> MHHHHHHHDGTEDPIHDRTSDYHKYLKVKQGDSDLFKLTVSDKRYIWYNPDPKERDSYECGEIVSETSDSFTFKTVDGQDRQVKKDDANQRNPIKFDGVEDMSELSYLNEPAVFHNLRVRYNQ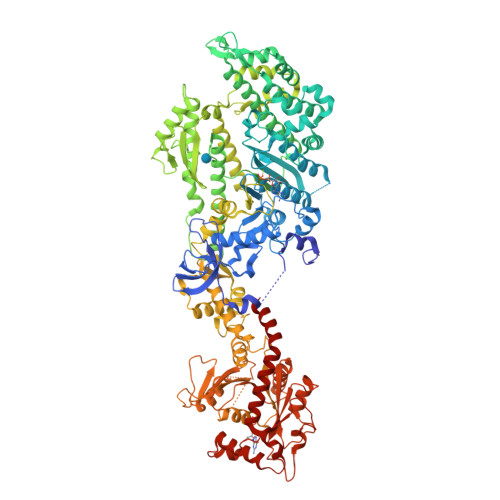DLIYTYSGLFLVAVNPFKRIPIYTQEMVDIFKGRRRNEVAPHIFAISDVAYRSMLDDRQNQSLLITGESGAGKTENTKKVIQYLASVAGRNQANGSGVLEQQILQANPILEAFGNAKTTRNNNSSRFGKFIEIQFNSAGFISGASIQSYLLEKSRVVFQSETERNYHIFYQLLAGATAEEKKALHLAGPESFNYLNQSGCVDIKGVSDSEEFKITRQAMDIVGFSQEEQMSIFKIIAGILHLGNIKFEKGAGEGAVLKDKTALNAASTVFGVNPSVLEKALMEPRILAGRDLVAQHLNVEKSSSSRDALVKALYGRLFLWLVKKINNVLCQERKAYFIGVLDISGFEIFKVNSFEQLCINYTNEKLQQFFNHHMFKLEQEEYLKEKINWTFIDFGLDSQATIDLIDGRQPPGILALLDEQSVFPNATDNTLITKLHSHFSKKNAKYEEPRFSKTEFGVTHYAGQVMYEIQDWLEKNKDPLQQDLELCFKDSSDNVVTKLFNDPNIASRAKKGANFITVAAQYKEQLASLMATLETTNPHFVRCIIPNNKQLPAKLEDKVVLDQLRCNGVLEGIRITRKGFPNRIIYADFVKRYYLLAPNVPRDAEDSQKATDAVLKHLNIDPEQYRFGITKIFFRAGQLARIEEAREQRISEITRGLVPRGSDQLIPVINKLQDVFNTLGSDPLDLPQIVVVGSQSSGKSSVLENIVGRDFLPRGSGIVTRRPLILQLTHLPIADDGSQTQEWGEFLHKPNDMFYDFSEIREEIIRDTDRMTGKNKGISAQPINLKIYSPHVVNLTLVDLPGITKVPVGDQPTDIEQQIRRMVMAYIKKQNAIIVAVTPANTDLANSDALQLAKEVDPEGKRTIGVITKLDLMDKGTDAMEVLTGRVIPLTLGFIGVINRSQEDIIAKKSIRESLKSEILYFKNHPIYKSIANRSGTAYLSKTLNKLLMFHIRDTLPDLKVKVSKMLSDVQGELSTY1-[4-[[4-[(5-cyclopentyl-1H-pyrazol-3-yl)amino]pyrimidin-2-yl]amino]phenyl]-3-[3-(trifluoromethyl)phenyl]urea 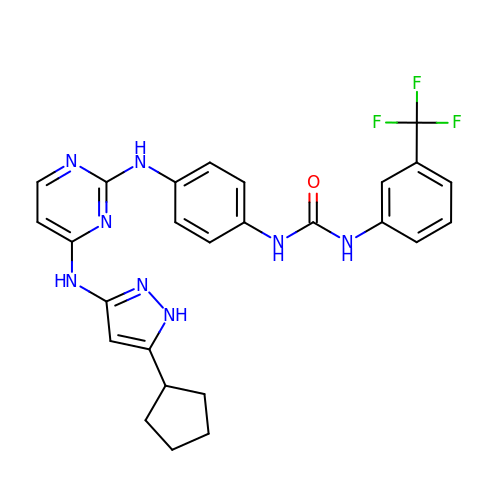| C26 H25 F3 N8 O | GBMIFBVLJSCVJT-UHFFFAOYSA-N> GSEMSVVEYEVVSKNLTSKMSHELLFSVKKRWFVKPFRHDRQLGKLHYKLLPGNYIAFGLYVLKNQDYARFEIAWVHVDKDGKIEERTVYSIETYWHIFIDIENDLNCPYVLA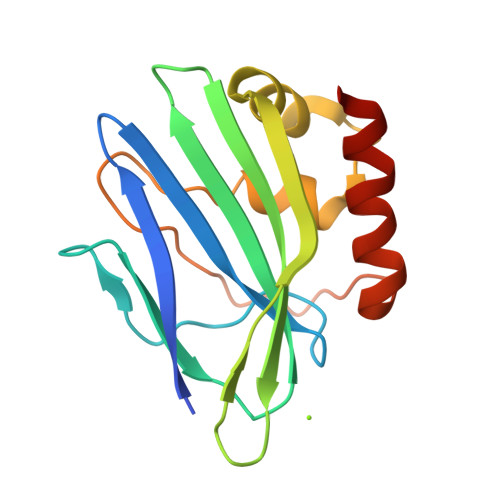KFIEMRPEFHKTAWVEESNYSIAEDDIQMVESIKRYLERKIASD> SMELITVHIVKGPMGFGFTIADSPGGGGQRVKQIVDSPR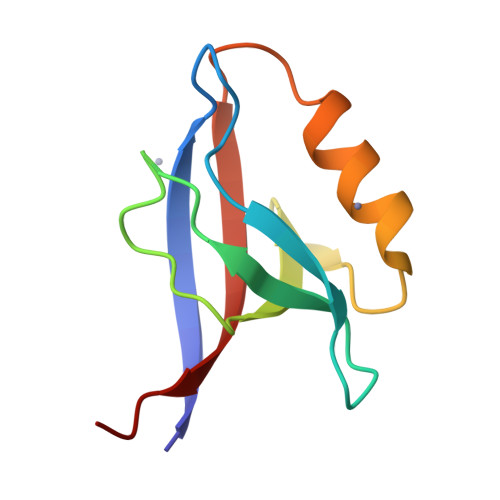SRGLKEGDLIVEVNKKNVQALTHNQVVDMLVESPKGSEVTLLVQRQTRL N-{5-[(3S)-3-{[5-(acetylamino)-1,3,4-thiadiazol-2-yl]amino}pyrrolidin-1-yl]-1,3,4-thiadiazol-2-yl}acetamide 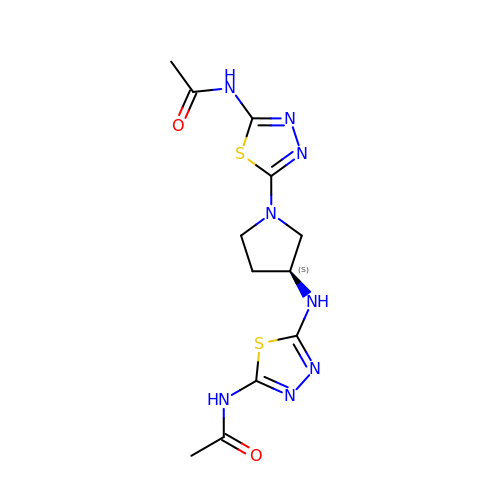| C12 H16 N8 O2 S2 | YVDVVIJXVARLFM-QMMMGPOBSA-N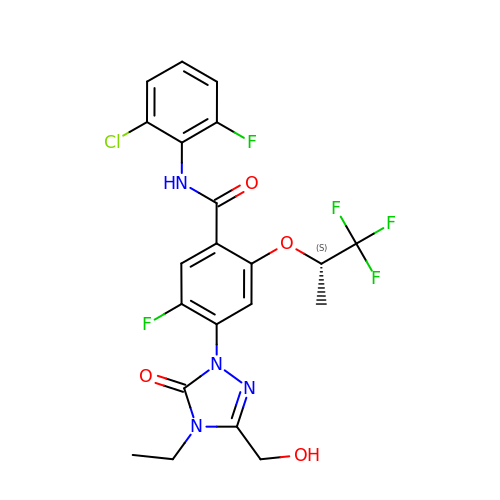~{N}-(2-chloranyl-6-fluoranyl-phenyl)-4-[4-ethyl-3-(hydroxymethyl)-5-oxidanylidene-1,2,4-triazol-1-yl]-5-fluoranyl-2-[(2~{S})-1,1,1-tris(fluoranyl)propan-2-yl]oxy-benzamide | C21 H18 Cl F5 N4 O4 | KNVJMHHAXCPZHF-JTQLQIEISA-N> 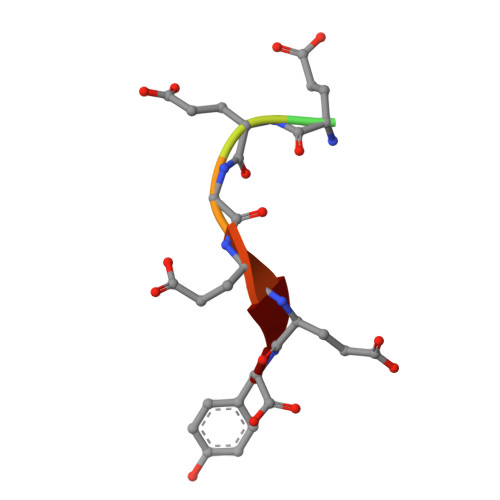GEEEGEEY>STRSTVPNDDGVENHGGGTLFVTVQRCRNLKNKETIGVSDPYVKLQLRKQTRKSPYISS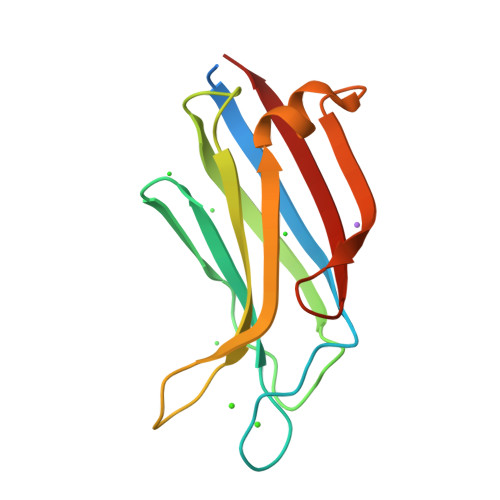TLNPDFNFEAALEVYDIRSDVLHISILDKNDLVKDRLMGTLRIMLSQVAAAPGDIIRGDMNLDPEGQISLELKLLRH[2x]>[2x]MVL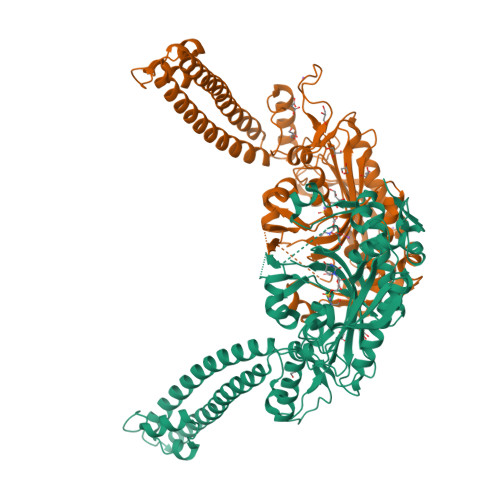DIQLFRDETGANIIRESQRRRFADPDIVDAIIEADKKWRRTQFLTEASKKLINICSKAVGAKKKAKEADGDTSEIPPQVKEAYENGTLKGEQVEQLCVLQLKQLSKDLSDQVAGLAKEAQQLEEERDKLMLNVGNILHESVPIAQDEETGNTVVRTFGNTTKRAKLNHVSIMERLGMMDTSKAVTSMAGGRSYVLKGGLVQLQVALVSYSLDFLVKRGYTPFYPPFFLNRDVMGEVAQLSQFDEELYQVSGDGDKKYLIATSEMPIAAYHRGRWFTELKEPLKYAGMSTCFRKEAGAHGRDTLGIFRVHQFDKIEQFVVCSPRQEESWRHLEDMITTSEEFNKSLGLPYRVVNICSGALNNAAAKKYDLEAWFPASGAFRELVSCSNCTDYQSQSVNCRYGPNLRGTAAQNVKEYCHMLNGTLCAITRTMCCICENYQTEEGVVIPDVLRPYMMGIEMIRFENNAQAEGTTPDKGE> MEDINFASLAPRHGTRPFMGTWNEIGTSQLNGGAFNW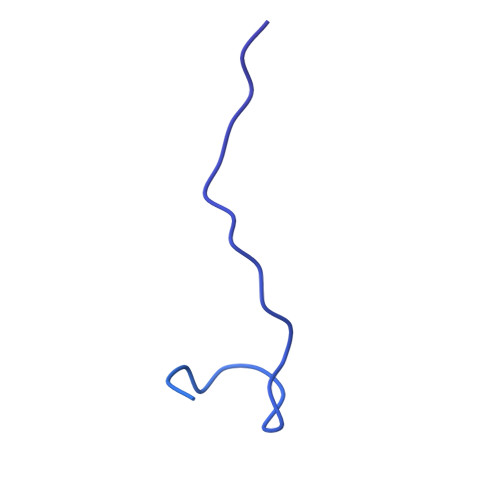SSVWSGLKNFGSTLRTYGNKAWNSSTGQLLREKLKDQNFQQKVVDGLASGINGVVDIANQAVQREINSRLDPRPPTVVEMEDATLPPPKGEKRPRPDAEETILQVDEPPSYEEAVKAGMPTTRIIAPLATGVMKPATLDLPPPPAPAPPKATPVVQAPPVATAVRRVPARRQAQNWQSTLHSIVGLGVKSLKRRRCY> GSSTNYGTIKWIFHALVFSYISFALISDKRYQKKEPLISSVHTKVKGIAEVKAEILENGMKKMVSGVFDTADYTFPLQGNSFFVMTNFIKTEGQQQGLCPDFPTARTICSSDRGCKKGRMDPQSKGIQTGRCVVYKERLKTCEVSAWCPIEEVKDAPRPALLNSAENFTVLIKNNIDFPGHNYTTRNILPGVNITCTFHKTQNPQCPIFRLGDIFQETGDSFSDVAIQGGIMGIEIYWDCNLDGWFHHCRPKYSFRRLDDKTTSESLYPGYNFRYAKYYKENNVEKRTLIKVFGIRFDILVFGTGGKFNVIQLAVYIGSVISYFGLATVFIDILINTYSASS

The P2X7 receptor, an extracellular ATP-gated ion channel predominantly expressed in immune cells of the blood and the brain, is an emerging target for treating refractory pain. P2X receptors are trimeric ligand-gated ion channels that facilitate extracellular-ATP mediated signaling along with the G protein-coupled P2Y receptors. For instance, the P2X7 receptor requires an unusually high concentration of ATP (EC50 ≥ 1 mM under physiological ion concentrations) for initial activation, its channel activity is facilitated by prolonged or repeated ATP applications, and it opens a membrane pore large enough for molecules up to ~900 Da to permeate. Here we identified and mapped the binding site for the P2X7 specific inhibitors for the first time using X-ray crystallography, and demonstrated by electrophysiological experiments that those inhibitors allosterically abrogate conformational changes associated with P2X7 receptor activation.

To define the structural basis for drug binding, we first sought to determine the crystal structures of a mammalian P2X7 receptor in the presence of five structurally distinct antagonists (A740003, A804598, AZ10606120, GW791343, and JNJ47965567). Surprisingly, all five structurally-unrelated compounds bind in the same pocket formed between neighboring subunits, which is juxtaposed with the ATP-binding pocket. This drug-binding pocket is surrounded by thirteen residues projecting mainly from β-strands (β4, β13 and β14) in the upper body domains of the neighboring subunits. Drug binding seems to be mediated mainly by hydrophobic interactions, especially at positions deep within the cavity, involving F95, F103, M105, F293, and V312. Despite structural diversity, all five P2X7 antagonists fit within the drug-binding pocket, highlighting that the size and the shape of the drug-binding pocket play major roles in determining the affinity and specificity of the drugs. Notably, drug-treated P2X7 receptor exhibited similar levels of fluorescence anisotropy, which drastically decreased in the presence of unlabeled-ATP. Together, these experiments strongly support that all five P2X7 antagonists are allosteric non-competitive inhibitors. Our data demonstrate that all five tested drugs are allosteric and non-competitive inhibitors, which is in contrast to the previous studies showing that A740003, A804598, and JNJ47965567 are competitive inhibitors.> MGSSHHHHHHSSGLVPRGSHSTQVAKKILVTCALPYANGSIHLGHMLEHIQADVWVRYQRMRGHEVNFICADDAHGTPIMLKAQQLGITPEQMIGEMSQEHQTDFAGFNISYDNYHSTHSEENRQLSELIYSRLKENGFIKNRTISQLYDPEKGMFLPDRFVKGTCPKCKSPDQYGDNCEVCGATYSPTELIEPKSVVSGATPVMRDSEHFFFDLPSFSEMLQAWTRSGALQEQVANKMQEWFESGLQQWDISRDAPYFGFEIPNAPGKYFYVWLDAPIGYMGSFKNLCDKRGDSVSFDEYWKKDSTAELYHFIGKDIIYFHSLFWPAMLEGSNFRKPSNLFVHGYVTVNGAKMSKSRGTFIKASTWLNHFDADSLRYYYTAKLSSRIDDIDLNLEDFVQRVNADIVNKVVNLASRNAGFINKRFDGVLASELADPQLYKTFTDAAEVIGEAWESREFGKAVREIMALADLANRYVDEQAPWVVAKQEGRDADLQAICSMGINLFRVLMTYLKPVLPKLTE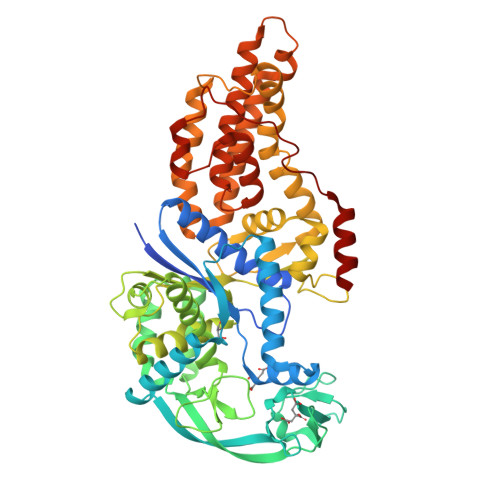RAEAFLNTELTWDGIQQPLLGHKVNPFKALYNRIDMRQVEALVEASK> MGFFDRLKAGLAKTRERLLKAIPWGGNLEEVLEELEMALLAADVGLSATEEILQEVRASGRKDLKEAVKEKLVGMLEPDERRATLRKLGFNPQKPKPVEPKGRVVLVVGVNGVGKTTTIAKLGRYYQNLGKKVMFCAGDTFRAAGGTQLSEWGKRLSIPVIQGPEGTDSAALAYDAVQAMKARGYDLLFVDTAGRLHTKHNLMEELKKVKRAIAKADPEEPKEVWLVLDAVTGQNGLEQAKKFHEAVGLTGVIVTKLDGTAKGGVLIPIVRTLKVPIKFVGVGEGPDDLQPFDPEAFVEALLED;> MFQQLSARLQEAIGRLRGRGRITEEDLKATLREIRRALMDADVNLEVTRDFVERVREEALGKQVLESLTPAEVILATVYEALKEALGGEARLPVLKDRNLWFLVGLQGSGKTTTAAKLALYYKGKGRRPLLVAADTQRPAAREQLRLLGEKVGVPVLEVMDGE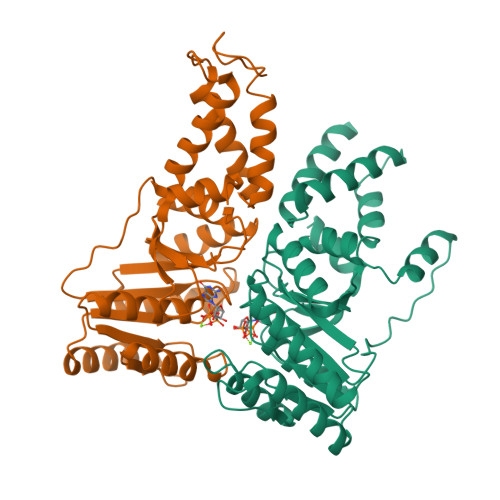SPESIRRRVEEKARLEARDLILVDTAGRLQIDEPLMGELARLKEVLGPDEVLLVLDAMTGQEALSVARAFDEKVGVTGLVLTKLDGDARGGAALSARHVTGKPIYFAGVSEKPEGLEPFYPERLAGRILGMGDVASL>[2x]MSHYKSNVRDQVFNLFEVFGVDKVLGADKFSDLDADTAREMLTEIARLAEGPIAESFVEGDRNPPVFDPETHTVTLPEGFKKSMRALFDGGWDKVGLAEHLGGIPMPRALQWALIEHILGANPAAYMYAMGPGMSEIFYNNGTDEQKKWATIAAERGWGATMVLTEPDAGSDVGAGRTKAVQQPDGTWHIEGVKRFITSADSDDLFENIMHLVLARPEGAGPGTKGLSLFFVPKFHFDHETGEIGERNGVFVTNVEHKMGLKVSATCELSLGQHGIPAVGWLVGEVHNGIAQMFDVIEQARMMVGTKAIATLSTGYLNALEYAKERVQGADMTQMTDKTAPRVTITHHPDVRRSLMTQKAYAEGLRAIYLYTATFQDAEVAQAVHGVDGDLAARVNDLLLPIVKGFGSET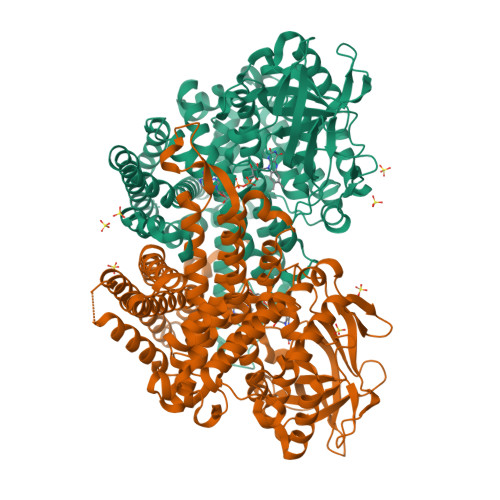AYAKLTESLQTLGGSGFLQDYPIEQYIRDSKIDSLYAGTTAIQAQDFFFRKIIRDKGQALAYVAGEIEQFIKNENGNGRLKTERELLATALADVQGMAASLTGYLMAAQEDAASIYKVGLGSVRFLMAVGDLLSGWLLARQAAVAIEKLDAGATGADKSFYEGKIAAASFFAKNMLPLLTSTRQIIENLDNDVMELDEAAF> KKADENKVKGEAFLTENKNKPGVVVLPSGLQYKVINSGNGVKPGKSDTVTVEYTGRLIDGTVFDSTEKTGKPATFQVSQVIPGWTEALQ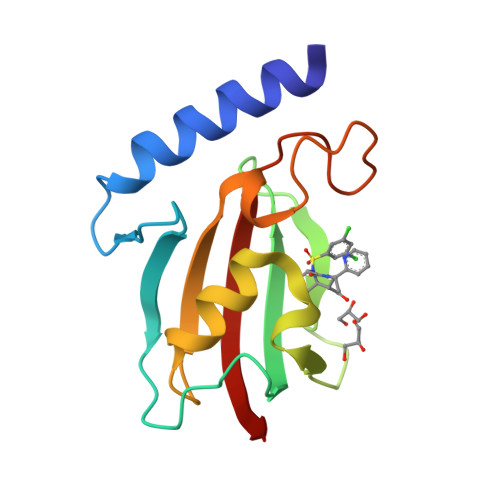LMPAGSTWEIYVPSGLAYGPRSVGGPIGPNETLIFKIHLISVKK(1-methyl-1H-indol-3-yl)acetic 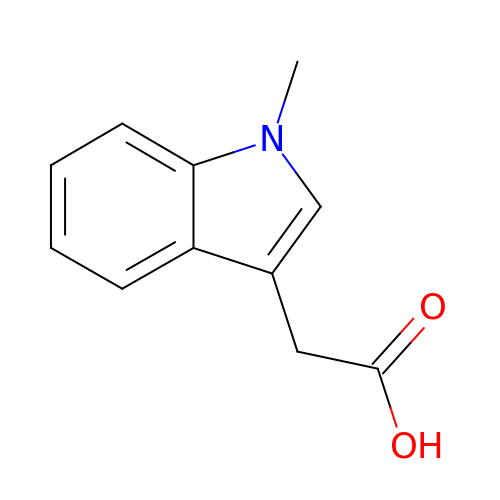acid | C11 H11 N O2 | NAIPEFIYIQFVFC-UHFFFAOYSA-N> XKPQPAVP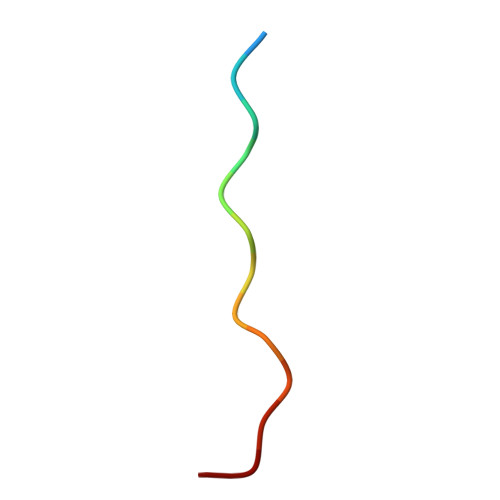PRPSAD>[4x]MQSDTQEVNDITTLANLHYNGSTPADAFEAEVTNILDRLNNNGIPINNKVACQFIMRGLSGEYRSLRYARSRCINMTVADLFLDIHAIYEEQQEWRRPLEH

Saccharomyces cerevisiae prevents uncontrolled retrotransposition of Ty1 subfamilies using distinct mechanisms: canonical Ty1 is inhibited by a self-encoded restriction factor, p22/p18, whereas Ty1’ is inhibited by an endogenized restriction factor, Drt2. The minimal inhibitory fragment of both restriction factors (p18m and Drt2m) is a conserved C-terminal capsid domain. Although the crystal structures of p18m and Drt2m are similar, three divergent residues found in a conserved hydrophobic interface direct restriction specificity. Structural and genetic analyses of p18m reveal that p18m and Ty1 Gag interact through a hydrophobic region that is shared between both proteins, termed the Dimer-1 interface. These observations suggest a lattice-poisoning model of restriction by p18m in which the CTD binds full-length Gag and forms dead-end intermediates in VLP assembly.

Ty1’ is not subject to the canonical CNC mechanism and is instead restricted by DRT2, a gene present at a fixed chromosomal locus that encodes the Ty1’ Gag CTD equivalent to p22. Drt2 also associates with Ty1’ Gag while forming VLPs and likely uses a lattice-poisoning mechanism to restrict retrotransposition. Therefore, we included F323S in Ty1’ CA-CTD constructs and in Drt2m F323S/Y329S (SS) for crystallographic analyses and F323S/Y326S/Y329S (SSS) for biophysical analyses. The asymmetric unit of wildtype and Ty1’ CA-CTD (F323S) crystals both contain two monomers arranged through a single Dimer-1 interface and the Drt2m(SS) crystals contain four Drt2m(SS) monomers arranged as two dimer-pairs through Dimer-1 interfaces. Further comparison of the p18m dimer with that of Drt2m(SS) reveals the strong similarity demonstrated by the 3D superposition of RMSD of 0.7 Å over 155 Cα backbone atoms. Inspection of the location of these divergent residues reveals that in p18m and Drt2m the three divergent residues lie at the center of the hydrophobic Dimer-1 interface. By contrast, in Drt2m and Ty1’ CA-CTD, it is the V266 sidechain on helix α1 that closely packs against F312 on helix α3 and because of the greater steric bulk of the V and F residues the distance between the V266 and F312 Cα atoms is increased to 6.8 Å. Concurrent with the increased spacing in the VTF interface of Drt2m and Ty1’ CA-CTD, the side chain of the conserved residue R315 can adopt a rotamer that allows it to swing in and hydrogen bond with T270 which is not possible with V270 in p18m. Thus, this “arginine-flip” mechanism provides a further level of discrimination and specificity between AVL and VTF Dimer-1 interfaces. Therefore, p18m(F323S) and Drt2m(SSS) form dimers in solution with sub-micromolar KD with some tendency for further p18m(F323S) self-association at higher concentration but that in Drt2m(SSS) is largely suppressed by the introduction of the triple serine mutation.> MESSVALKGNDFVIIGTDSSVKNSYLVLKREEDKFYNINNKVVFTYLGDQGDAFRTSSFINEKLVYEEIQNNVEITPKVTANVIQKTLYDNLRSHPKNCYFLVGGLSQDGPELYSVDLYGSLHENDFMAVGISTYFCYGVLDKEYHKNITKEDGIKI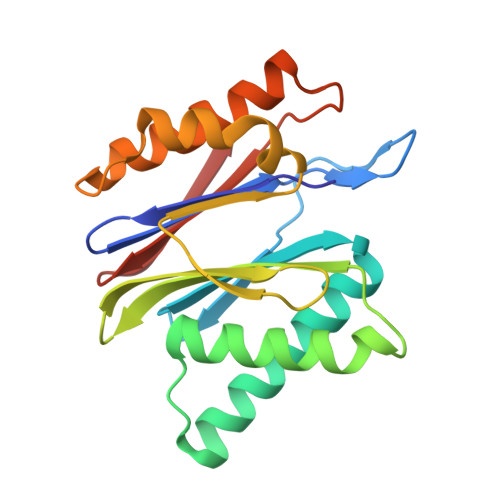IQKCFDVLKQRCSVDISNIEIKIVSKEGVETINKVL>[2x]EAPYASLTEIEHLVQSVCKSYRETCQLRLEDLLRQRSNIFSREEVTGYQRKSMWEMWERCAHHLTEAIQYVVEFAKRLSGFMELCQNDQIVL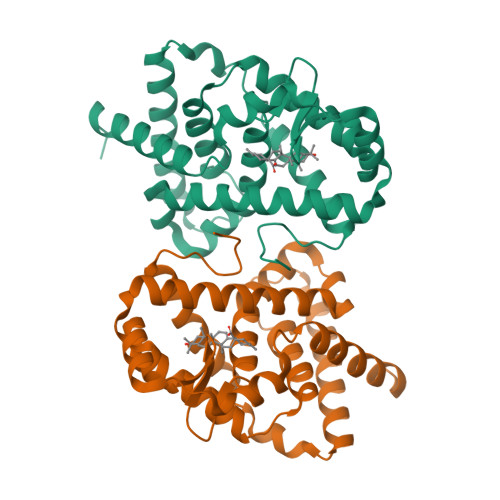LKAGAMEVVLVRMCRAYNADNRTVFFEGKYGGMELFRALGCSELISSIFDFSHSLSALHFSEDEIALYTALVLINAHRPGLQEKRKVEQLQYNLELAFHHHLCKTHRQSILAKLPPKGKLRSLCSQHVERLQIFQHLHPIVVQAAFPPLYKELFSTETESPVGLSK>[4x]ILVEGDGIPPPIKSFKEMKFPAAILRGLKKKGIHHPTPIQIQGIPTILSGRDMIGIAFTGSGKTLVFTLPVIMFCLEQEKRLPFSKREGPYGLIICPSRELARQTHGILEYYCRLLQEDSSPLLRCALCIGGMSVKEQMETIRHGVHMMVATPGRLMDLLQKKMVSLDICRYLALDEADRMIDMGFEGDIRTIFSYFKGQRQTLLFSATMPKKIQNFAKSALVKPVTINVG

In contrast, DEAD box protein 41 (DDX41), a member of the helicase superfamily 2 (SF2), is unique in that it can recognize two different types of ligands, double-stranded DNA (dsDNA) and CDN45. DDX41 consists of two RecA-like domains (i.e., DEAD and HELICc domains), which are conserved among DEAD box proteins. These domains have several conserved motifs, such as the Q motif and motif I, which are both essential for ATP binding by the DEAD box proteins. In this work, we determined two different crystal structures of the DDX41 DEAD domain in apo forms.

We determined the apo-form structures of two constructs, residues 169–402 (DEAD402) and 169–399 (DEAD399), at 1.5 and 2.2 Å resolutions, respectively. In contrast to DEAD402, the crystal structure of DEAD399 contains four molecules in the asymmetric unit, and their N-terminal regions adopt two different conformations. In one conformation, the Q motif is located away from α3 and motif I. Helix α2 is rearranged to form two β strands (β1′ and β2′), and residues 169–183 are disordered. We hereafter refer to this conformation of the N-terminal region as the “open form 1”. In the other conformation, helix α3 and motif I adopt similar conformations to those in open form 1, while residues 169–209, including the entire Q motif, are disordered. We hereafter refer to this conformation of the N-terminal region as the “open form 2”. In these models, the Q motif, including Ile201 and Gln208, is distant from the modeled ATP in the open form 1, while it is disordered in the open form 2. Moreover, in both open forms 1 and 2, motif I forms part of the extended α3 helix, which sterically clashes with the modeled ATP. Consequently, the structure of the ATP-binding site is completely rearranged in these open forms, and thus they do not seem to be able to bind ATP. Therefore, these results suggested that the closed form represents the ATP-bound state of DDX41, while both open forms 1 and 2 represent its nucleotide-free state.>[2x]HHHHHHHHGSGAGWSHPQFEKGGSGLVPRGS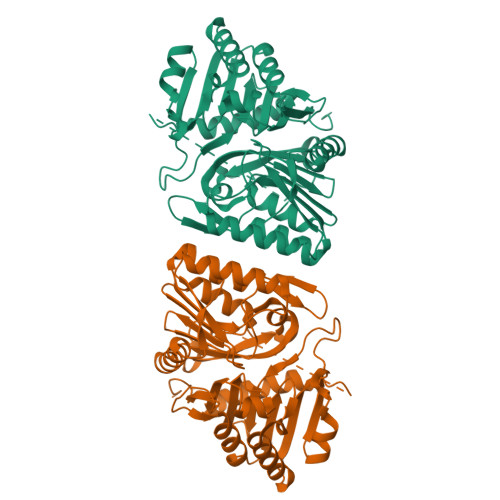GSVPAGAKCRLVETLPENMDFRSDHLTTFECFNEIITLAKKYIYIASFCCNPLSTTRGALIFDKLKEASEKGIKIIVLLDERGKRNLGELQSHCPDINFITVNIDKKNNVGLLLGCFWVSDDERCYVGNASFTGGSIHTIKTLGVYSDYPPLATDLRRRFDTFKAFNSAKNSAANLASAAAALPVSTAYHIKNPIGGVFFTDSPEHLLGYSRDLDTDVVIDKLKSAKTSIDIEHLAIVPTTRVDGNSYYWPDIYNSIIEAAINRGVKIRLLVGNWDKNDVYSMATARSLDALCVQNDLSVKVFTIQNNTKLLIVDDEYVHITSANFDGTHYQNHGFVSFNSIDKQLVSEAKKIFERDWVSSHSKSLKI>[2x]GSAKDPMKGLTELLKGSLEGMILERISR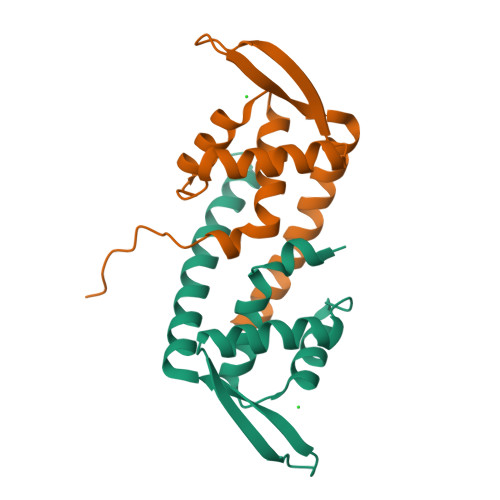GETYGYEITKYLNDLGFDEIVEGTVYTILVRLEKKGLVEIEKKKSELGPPRKFYTLSPAGEEELAIFWKRWDFIQGKIMQVKGGQA> MKKLIPILEKIPEVELPVKEITFKEKLKWTGIVLVLYFIMGCIDVYTAGAQI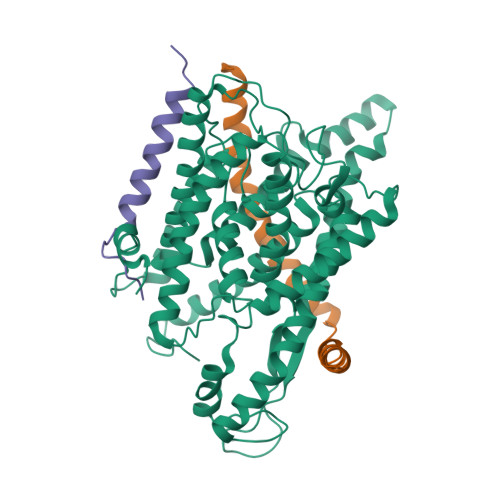PAIFEFWQTITASRIGTLITLGIGPIVTAGIIMQLLVGSGIIQMDLSIPENRALFQGCQKLLSIIMCFVEAVLFVGAGAFGILTPLLAFLVIIQIAFGSIILIYLDEIVSKYGIGSGIGLFIAAGVSQTIFVGALGPEGYLWKFLNSLIQGVPNIEYIAPIIGTIIVFLMVVYAECMRVEIPLAHGRIKGAVGKYPIKFVYVSNIPVILAAALFANIQLWGLALYRMGIPILGHYEGGRAVDGIAYYLSTPYGLSSVISDPIHAIVYMIAMIITCVMFGIFWVETTGLDPKSMAKRIGSLGMAIKGFRKSEKAIEHRLKRYIPPLTVMSSAFVGFLATIANFIGALGGGTGVLLTVSIVYRMYEQLLREKVSELHPAIAKLLNK;> MKTDFNQKIEQLKEFIEECRRVWLVLKKPTKDEYLAVAKVTALGISLLGIIGYIIHVPATYIKGILKPPTTPRV;> MSKREETGLATSAGLIRYMDETFSKIRVKPEHVIGVTVAFVIIEAILTYGRFL>MTSQTPTRKPRARDLGLPFTGVTGPYNAITDVDGVGVGFQTII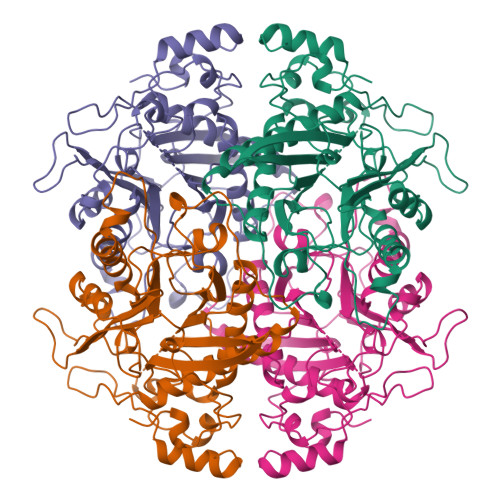ENEPRPGRKRPARSGVTAILPHMQSETPVPVYAGVHRFNGNGEMTGTHWIEDGGYFLGPVVITNTHGIGMAHHATVRWMVDRYASTYQTDDFLWIMPVVAETYDGALNDINGFPVTEADVRKALDNVASGPVQEGNCGGGTGMITYGFKGGTGTASRVVEFGGRSFTIGALVQANHGQRDWLTIAGVPVGQHMRDGTPQSQLQERGSIIVVLATDLPLMPHQLKRLARRASIGIGRNGTPGGNNSGDIFIAFSTANQRPMQHRSAPFLDVEMVNDEPLDTVYLAAVDSVEEAVVNAMIAAEDMGGTPFDRLLVQAIDHERLRAVLRQYGRLA[6x]1-(4-CYANO-PHENYL)-3-[2-(2,6-DICHLORO-PHENYL)-1-IMINO-ETHYL]-THIOUREA | C16 H12 Cl2 N4 S | 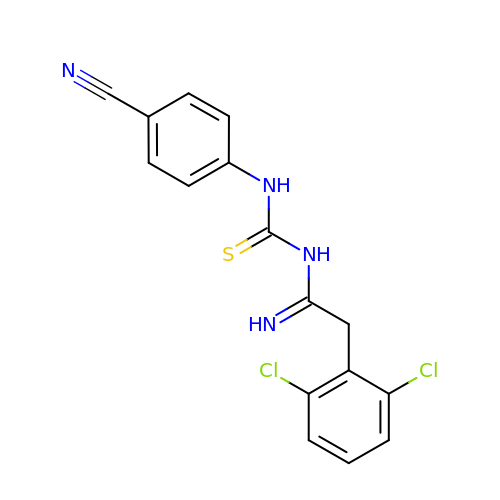NWKJBFSBEAMDBE-UHFFFAOYSA-N In our studies we have focused on the periplasmic segment of GspL (historically called XcpY) from P. aeruginosa, GspLperi, which consists of two domains: a membrane proximal domain (MPD) connected via a short linker to a ferredoxin-like domain (FLD). The inner-membrane bitopic protein GspL can be considered a central player in the T2SS because it appears to interact extensively with other components of the system. Even though the exact mode of secretion via T2SS has not been fully elucidated, the role of GspL is anticipated to help in linking adenosine triphosphate (ATP) hydrolysis to the assembly of the pseudopilus, which together constitute the two crucial steps in exoprotein transport. In this work we presented two distinct crystal structures of GspLfld, which in combination with the crystal structure of GspLfld from Vibrio parahaemolyticus, provide direct evidence for the conservation of a hydrophobic dimer interface.

The continuity of the strand β1 of crystal form 1 is compromised due to the adoption by Leu327 of two distinct conformations, with only one of them providing extension of the strand. The core of the dimer interaction interface of crystal form 1 of GspLfld is almost purely hydrophobic. On the α1 side, close to the N-terminus of the helix, the side chains of Leu306 and Ala313′ establish a heterotypic interaction which is complemented by Ile316′. On the opposite side of the interface another hydrophobic clamp is formed by Phe329, Leu327a′ and Val324′, the residues belonging to strand β1. The core of the interface is constituted by two interactions between symmetry related residues: the first involving Leu309 and the second involving b-conformers of Leu327 (bottom panel seen clockwise from top left). The distance between the main chain atoms of β1 and β1′ of crystal form 1 is in the range of 4.5–5.0 Å and is drastically greater than the equivalent interdomain in crystal form 2, which are instead within hydrogen bonding distances (2.8–3.0 Å). The electron density of the inter-strand region of crystal form 1 has revealed the presence of an ordered water molecule positioned halfway between the main chain nitrogen of Leu327 and the carbonyl oxygen of Phe329′ (red sphere). In this regard, crystal form 2 and the V. parahaemolyticus crystal form of GspLfld appear as closed versions of the dimer whereas crystal form 1 exploits a novel conformation, resulting in an open variant of the interface. Nevertheless, the GspLfld dimer is capable of subtle opening of the interface, which does not affect its hydrophobic core but perturbs extension of antiparallel β-sheet, as documented by crystal form 1.

> GQLLGLLGQAATVIGGEPTVSVEQLDFSAARGDVALQVRAPGFDVLERLRSRLSESGLAVQLGSASRDGSTVSARLVIGG>SVTVKRIIDNTVIVPKLPANEDPVEYPADYFRKSKEIPLYINTTKSLSDLRGYVYQGLKSGNVSIIHVNSYLYGALKDIRGKLDKDWSSFGINIGKAGDTIGIFDLVSLKALDGVLPDGVSDASRTSADDKWLPLYLLGLYRVGRTQMPEYRKKLMDGLTNQCKMINEQFEPLVPEGRDIFDVWGNDSNYTKIVAAVDMFFHMFKKHECASFRYGTIVSRFKDCAALATFGHLCKITGMSTEDVTTWILNREVADEMVQMMLPGQEIDKADSYMPYLIDFGLSSKSPYSSVKNPAFHFWGQLTALLLRSTRARNARQPDDIEYTSLTTAGLLYAYAVGSSADLAQQFCVGDNKYTPDDSTGGLTTNAPPQGRDVVEWLGWFEDQNRKPTPDMMQYAK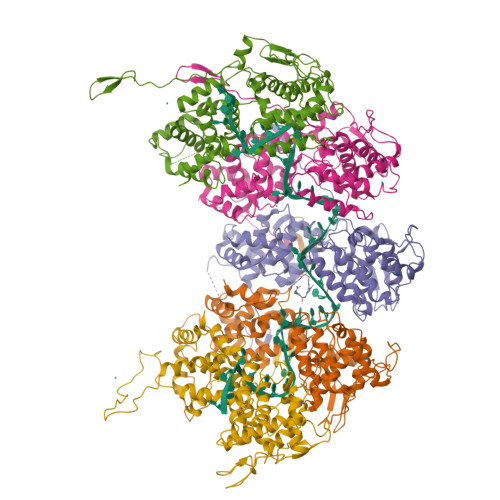RAVMSLQGLREKTIGKYAKSEFDK[5x]> MDYKDHDGDYKDHDIDYKDDDDKMSLTEQIEQFASRFRDDDATLQSRYSTLSELYDIMELLNSPEDYHFFLQAVIPLLLNQLKEVPISYDAHSPEQKLRNSMLDIFNRCLMNQTFQPYAMEVLEFLLSVLPKENEENGILCMKVLTTLFKSFKSILQDKLDSFIRIIIQIYKNTPNLINQTFYEAGKAEQGDLDSPKEPQADELLDEFSKNDEEKDFPSKQSSTEPRFENSTSSNGLRSSMFSFKILSECPITMVTLYSSYKQLTSTSLPEFTPLIMNLLNIQIKQQQEAREQAESRGEHFTSISTEIINRPAYCDFILAQIKATSFLAYVFIRGYAPEFLQDYVNFVPDLIIRLLQDCPSELSSARKELLHATRHILSTNYKKLFLPKLDYLFDERILIGNGFTMHETLRPLAYSTVADFIHNIRSELQLSEIEKTIKIYTGYLLDESLALTVQIMSAKLLLNLVERILKLGKENPQEAPRAKKLLMIIIDSYMNRFKTLNRQYDTIMKYYGRYETHKKEKAEKLKNSIQDNDKESEEFMRKVLEPSDDDHLMPQPKKEDINDSPDVEMTESDKVVKNDVEMFDIKNYAPILLLPTPTNDPIKDAFYLYRTLMSFLKTIIHDLKVFNPPPNEYTVANPKLWASVSRVFSYEEVIVFKDLFHECIIGLKFFKDHNEKLSPETTKKHFDISMPSLPVSATKDARELMDYLAFMFMQMDNATFNEIIEQELPFVYERMLEDSGLLHVAQSFLTSEITSPNFAGILLRFLKGKLKDLGNVDFNTSNVLIRLFKLSFMSVNLFPNINEVVLLPHLNDLILNSLKYSTTAEEPLVYFYLIRTLFRSIGGGRFENLYRSIKPILQVLLQSLNQMILTARLPHERELYVELCITVPVRLSVLAPYLPFLMKPLVFALQQYPDLVSQGLRTLELCIDNLTAEYFDPIIEPVIDDVSKALFNLLQPQPFNHAISHNVVRILGKLGGRNRQFLKPPTDLTEKTELDIDAIADFKINGMPEDVPLSVTPGIQSALNILQSYKSDIHYRKSAYKYLTCVLLLMTKSSAEFPTNYTELLKTAVNSIKLERIGIEKNFDLEPTVNKRDYSNQENLFLRLLESVFYATSIKELKDDAMDLLNNLLDHFCLLQVNTTLLNKRNYNGTFNIDLKNPNFMLDSSLILDAIPFALSYYIPEVREVGVLAYKRIYEKSCLIYGEELALSHSFIPELAKQFIHLCYDETYYNKRGGVLGIKVLIDNVKSSSVFLKKYQYNLANGLLFVLKDTQSEAPSAITDSAEKLLIDLLSITFADVKEEDLGNKVLENTLTDIVCELSNANPKVRNACQKSLHTISNLTGIPIVKLMDHSKQFLLSPIFAKPLRALPFTMQIGNVDAITFCLSLPNTFLTFNEELFRLLQESIVLADAEDESLSTNIQKTTEYSTSEQLVQLRIACIKLLAIALKNEEFATAQQGNIRIRILAVFFKTMLKTSPEIINTTYEALKGSLAENSKLPKELLQNGLKPLLMNLSDHQKLTVPGLDALSKLLELLIAYFKVEIGRKLLDHLTAWCRVEVLDTLFGQDLAEQMPTKIIVSIINIFHLLPPQADMFLNDLLLKVMLLERKLRLQLDSPFRTPLARYLNRFHNPVTEYFKKNMTLRQLVLFMCNIVQRPEAKELAEDFEKELDNFYDFYISNIPKNQVRVVSFFTNMVDLFNTMVITNGDEWLKKKGNMILKLKDMLNLTLKTIKENSFYIDHLQLNQSIAKFQALYLRFTELSERDQNPLLLDFIDFSFSNGIKASYSLKKFIFHNIIASSNKEKQNNFINDATLFVLSDKCLDARIFVLKNVINSTLIYEVATSGSLKSYLVEDKKPKWLELLHNKIWKNSNAILAYDVLDHHDLFRFELLQLSAIFIKADPEIIAEIKKDIIKFCWNFIKLEDTLIKQSAYLVTSYFISKFDFPIKVVTQVFVALLRSSHVEARYLVKQSLDVLTPVLHERMNAAGTPDTWINWVKRVMVENSSSQNNILYQFLISHPDLFFNSRDLFISNIIHHMNKITFMSNSNSDSHTLAIDLASLILYWENKTLEITNVNNTKTDSDGDVVMSDSKSDINPVEADTTAIIVDANNNSPISLHLREACTAFLIRYVCASNHRAIETELGLRAINILSELISDKHWTNVNVKLVYFEKFLIFQDLDSENILYYCMNALDVLYVFFKNKTKEWIMENLPTIQNLLEKCIKSDHHDVQEALQKVLQVIMKAIKAQGVSVIIEEESPGKTFIQMLTSVITQDLQETSSVTAGVTLAWVLFMNFPDNIVPLLTPLMKTFSKLCKDHLSISQPKDAMALEEARITTKLLEKVLYILSLKVSLLGDSRRPFLSTVALLIDHSMDQNFLRKIVNMSRSWIFNTEIFPTVKEKAAILTKMLAFEIRGEPSLSKLFYEIVLKLFDQEHFNNTEITVRMEQPFLVGTRVEDIGIRKRFMTILDNSLERDIKERLYYVIRDQNWEFIADYPWLNQALQLLYGSFNREKELSLKNIYCLSPPSILQEYLPENAEMVTEVNDLELSNFVKGHIASMQGLCRIISSDFIDSLIEIFYQDPKAIHRAWVTLFPQVYKSIPKNEKYGFVRSIITLLSKPYHTRQISSRTNVINMLLDSISKIESLELPPHLVKYLAISYNAWYQSINILESIQSNTSIDNTKIIEANEDALLELYVNLQEEDMFYGLWRRRAKYTETNIGLSYEQIGLWDKAQQLYEVAQVKARSGALPYSQSEYALWEDNWIQCAEKLQHWDVLTELAKHEGFTDLLLECGWRVADWNSDRDALEQSVKSVMDVPTPRRQMFKTFLALQNFAESRKGDQEVRKLCDEGIQLSLIKWVSLPIRYTPAHKWLLHGFQQYMEFLEATQIYANLHTTTVQNLDSKAQEIKRILQAWRDRLPNTWDDVNMWNDLVTWRQHAFQVINNAYLPLIPALQQSNSNSNINTHAYRGYHEIAWVINRFAHVARKHNMPDVCISQLARIYTLPNIEIQEAFLKLREQAKCHYQNMNELTTGLDVISNTNLVYFGTVQKAEFFTLKGMFLSKLRAYEEANQAFATAVQIDLNLAKAWAQWGFFNDRRLSEEPNNISFASNAISCYLQAAGLYKNSKIRELLCRILWLISIDDASGMLTNAFDSFRGEIPVWYWITFIPQLLTSLSHKEANMVRHILIRIAKSYPQALHFQLRTTKEDFAVIQRQTMAVMGDKPDTNDRNGRRQPWEYLQELNNILKTAYPLLALSLESLVAQINDRFKSTTDEDLFRLINVLLI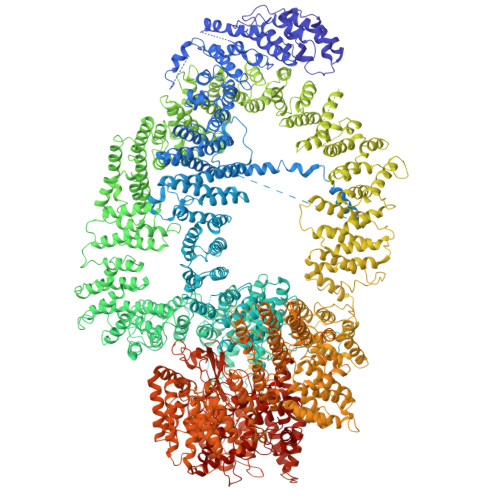DGTLNYNRLPFPRKNPKLPENTEKNLVKFSTTLLAPYIRPKFNADFIDNKPDYETYIKRLRYWRRRLENKLDRASKKENLEVLCPHLSNFHHQKFEDIEIPGQYLLNKDNNVHFIKIARFLPTVDFVRGTHSSYRRLMIRGHDGSVHSFAVQYPAVRHSRREERMFQLYRLFNKSLSKNVETRRRSIQFNLPIAIPLSPQVRIMNDSVSFTTLHEIHNEFCKKKGFDPDDIQDFMADKLNAAHDDALPAPDMTILKVEIFNSIQTMFVPSNVLKDHFTSLFTQFEDFWLFRKQFASQYSSFVFMSYMMMINNRTPHKIHVDKTSGNVFTLEMLPSRFPYERVKPLLKNHDLSLPPDSPIFHNNEPVPFRLTPNIQSLIGDSALEGIFAVNLFTISRALIEPDNELNTYLALFIRDEIISWFSNLHRPIIENPQLREMVQTNVDLIIRKVAQLGHLNSTPTVTTQFILDCIGSAVSPRNLARTDVNFMPWF>[2x]GPHMLEI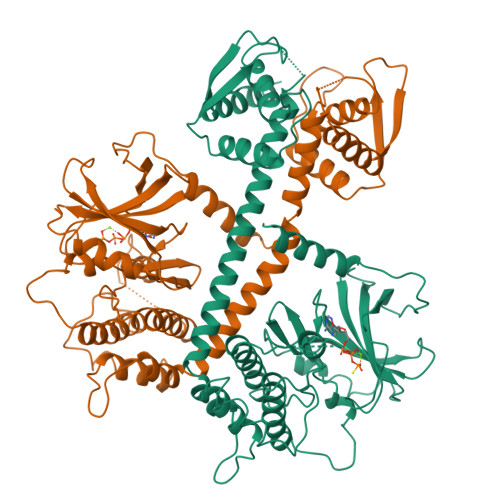PKDRRENLQKKLFHMQQLLPNSGLPNLDRWHSLFPLDTKATRNSTCFGYPSWMYKAQNNKNGRHFALRRIEGYRLTNEKAILNVTKEWKKIINANIVTVHEAFTTEFFGDSSLIFVYDFHPLSETLYDHHFPPNNSHNRLRNTNKIPENLLWSYVCQIANALLAIHNAKLAARCLELSKIIWENNRIRLAACSILDVLHHDSPNRKTIEELQQEDFVKFGRIILALATNTPTLNFNNIDAALATIVPRYSTQLRGVLEWLIKPSAPGETKTVETLMPMIGARFANFANFVMQESDEKEFHLMRELENGRIARLMFKLSVVNERGDSCGVHNWSETGERLLLKLFRDYVFHQVDADGKARLDTNHYLNCLSKLDASSEEQILLTSRDNATVFVVSYRSIRQMLDRAYGELGKESKPSATGATI Since ENPP1 is part of the highly conserved nucleotide pyrophosphatase/phosphodiesterase (NPP) protein family, we investigated the evolutionary conservation of the analogous histidine residue and its requirement for cGAMP degradation. Two zinc ions are required for NPP’s catalytic activity, with Zn1 being particularly important for stabilizing the leaving group, whereas Zn2 activates the threonine nucleophile. We found that Xac NPP not only degrades cyclic dinucleotides but also prefers 2′-5′–linked over 3′-5′–linked cyclic dinucleotides. Furthermore, the conserved histidine is required for degrading the 2′-5′ but not 3′-5′ phosphodiester linkage.

Since the histidine (H362 in mouse ENPP1 and H214 in Xac NPP) is one of three residues that chelates Zn1, we hypothesized that the loss of the histidine prevents Zn1 binding. Indeed, in contrast to Xac NPPWT, which binds two zincs, our 2.0 Å crystal structure revealed that Xac NPPH214A was missing Zn1. We found that Xac NPPWT degrades ATP and that Xac NPPH214A (which corresponds to the mouse H362A mutation) degrades ATP several-fold faster than NPPWT, suggesting that H214 is not conserved for the purpose of scavenging base products from ATP. Indeed, Xac NPPWT degrades the metazoan 2′3′-cGAMP while the NPPH214A mutant does not, mirroring our findings with mouse ENPP1H362A. Interestingly, H214 is required to cleave cyclic dinucleotides with 2′-5′ linkages (2′3′-cGAMP, 3′2′-cGAMP, 2′3′-CDA, 2′3′-CDG), but is not required for cyclic dinucleotides with only 3′-5′ linkages (3′3′-cGAMP, 3′3-CDA, or 3′3-CDG). We also docked 3′3′-cGAMP and 2′3′-cGAMP into our H214A Xac NPP structure. Similar to ATP, the free 2′-OH group in 3′3′-cGAMP can also take the place of the missing histidine to chelate Zn1 while the free 3′-OH group in 2′3′-cGAMP is too far away from Zn1. We propose that ATP and 3′-5′–linked cyclic dinucleotides are able to compensate for the loss of histidine with their γ-phosphate oxygen and 2′-OH group, respectively, explaining why H362 in mouse ENPP1 and H214 in Xac NPP are only required for cleaving 2′-5′–linked phosphodiester bonds.

>[2x]TPHALLLISIDGLRADMLDRGITPNLSHLAREGVRARWMAPSYPSLTFPNHYTLVTGLRPDHHGIVHNSMRDPTLGGFWLSKSEAVGDARWWGGEPVWVGVENTGQHAATWSWPGSEAAIKGVRPSQWRHYQKGVRLDTRVDAVRGWLATDGAQRNRLVTLYFEHVDEAGADHGPESRQYADAVRAVDAAIGRLLAGMQRDGTRARTNIIVVSDHGMAEVAPGHAISVEDIAPPQIATAITDGQVIGFEPLPGQQAAAEASVLGAHDHYDCWRKAELPARWQYGSHPRIPSLVCQMHEGWDALFPDKLAKRAQRGTRGSHGYDPALPSMRAVFLAQGPDLAQGKTLPGFDNVDVYALMSRLLGIPAAPNDGNPATLLPALRMP>MTNFVPTPSVPAPDIVRCAYMEIVVTDLAKSREFYVDVLGLHVTEEDENTIYLRSLEEFIHHNLVLRQGPIAAVAAFAYRVKSPAEVDAAEAYYKELGCRTERRKEGFTKGIGDSVRVEDPLGFPYEFFYETEHVERLTQRYDLYSAGELVRLDHFNQVTPDVPRGRAYLEDLGFRVSEDIKDSDGVTYAAWMHRKQTVHDTALTGGNGPRMHHVAFATHEKHNIIQICDKMGALRISDRIERGPGRHGVSNAFYLYILDPDGHRIEIYTQDYYT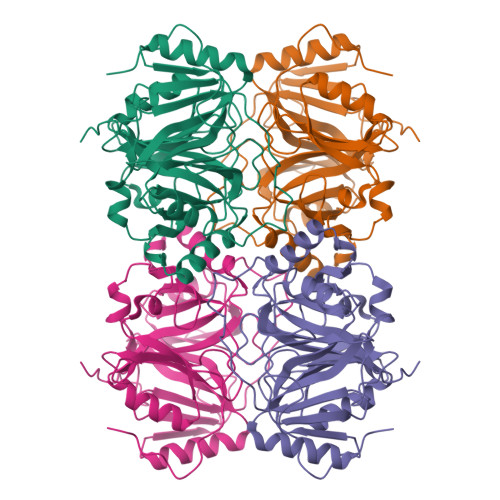GDPDNPTITWDVHDNQRRDWWGNPVVPSWYTEASLVLDLDGNPQPVIV[2x]>MLVTGLEILRKARAEGYGVGAFNTNNMEFTQAILEAAEEMKSPVILALSEGAMKYGGRALTRMVVALAQEARVPVAVHLDHGSSYESVLKALREGFTSVMIDKSHEDFETNVRETKRVVEAAHAVGVTVEAELGRLA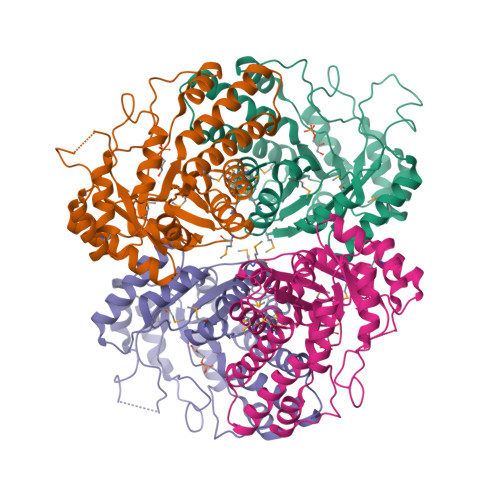GIEEHVAVDEKDALLTNPEEARIFMERTGADYLAVAIGTSHGAYKGKGRPFIDHPRLARIAKLVPAPLVLHGASAVPQELVERFRAAGGEIGEASGIHPEDIKKAISLGIAKINTDTDLRLAFTALVRETLGKNPKEFDPRKYLGPAREAVKEVVKSRMELFGSVGRA[4x]>[2x]TYTTRQIGAKNTLEYKVYIEKDGKPVSAFHDIP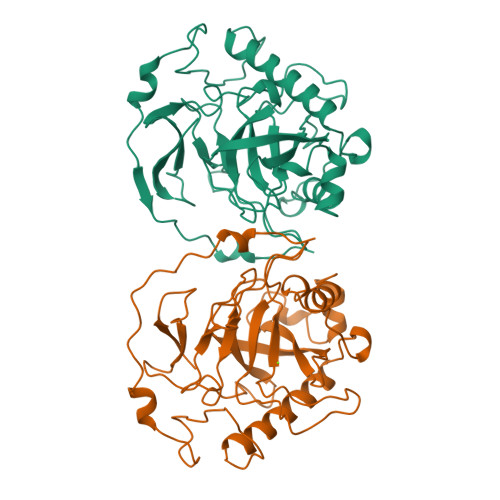LYADKENNIFNMVVEIPRWTNAKLEITREETLNPIIQDTKKGKLRFVRNCFPHHGYIHNYGAFPQTWEDPNVSHPETKAVGDNDPIDVLEIGETIAYTGQVKQVKALGIMALLDEGETDWKVIAIDINDPLAPKLNDIEDVEKYFPGLLRATNEWFRIYKIPDGKPENQFAFSGEAKNKKYALDIIKETHDSWKQLIAGKSSDSKGIDLTNVTLPDTPTYSKAASDAIPPASLKADAPIDKSIDKWFF> EAEAEFATPALRFVAVGDWGGVPNAPFHTAREMANAKEIARTVQILGADFILSLGDNFYFTGVQDINDKRFQETFEDVFSDRSLRKVPWYVLAGNHDHLGNVSAQIAYSKISKRW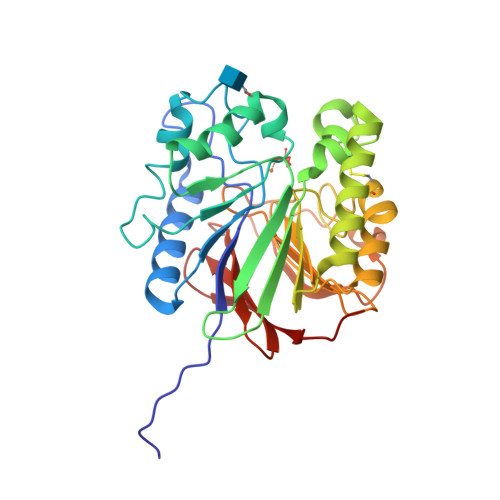NFPSPFYRLHFKIPQTNVSVAIFMLDTVTLCGNSDDFLSQQPERPRDVKLARTQLSWLKKQLAAAREDYVLVAGHYPVWSIAEHGPTHCLVKQLRPLLATYGVTAYLCGHDHNLQYLQDENGVGYVLSGAGNFMDPSKRHQRKVPNGYLRFHYGTEDSLGGFAYVEISSKEMTVTYIEASGKSLFKTRLPRRARP>[2x]SVGKEKKSRILTKPCVIEYEGQIVGYGSKELRVETIS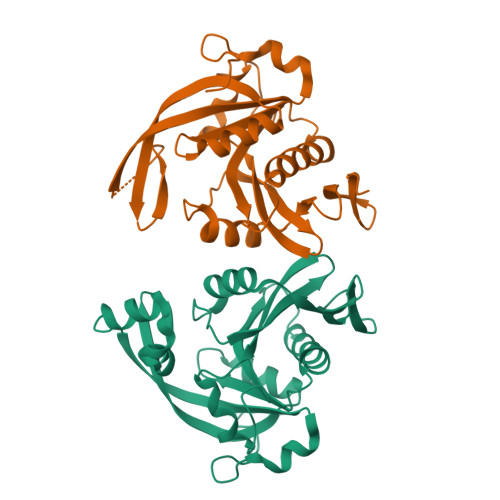CWLARTIIQTKHYSRRFVNNSYLHLGVFSGRDLVGVLQWGYALNPNSGRRVVLETDNRGYMELNRMWLHDDMPRNSEARAISYALKVIRLLYPSVEWVQSFADERCGRAGVVYQASNFDFIGSHESTFYELDGEWYHEITMNAIKRGGQRGVYLRANKERAVVHKFNQYRYIRFLNKRARKRLNTKLFKVQPYPK> QGGPWTPA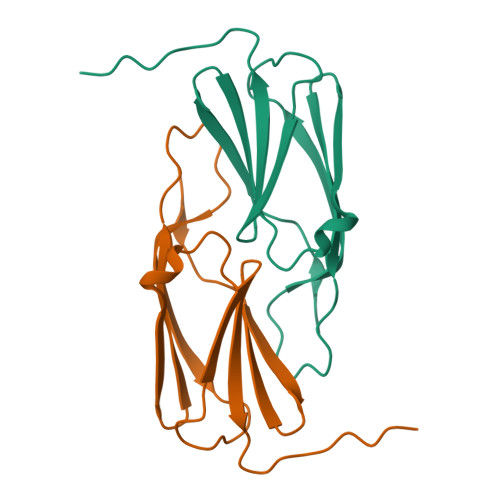ADWRDAGTHLDLLLDVPGVDAGTLALAEDGGQLTVSGERPGTEHLLRSERPSGRFVRELAFPEPVRPASGVASLAGGVLTVRFEKLRPTIDVTA> SITSSLDVRPEIKQAVTVRPGMCGPGSLFVGQLGDWTWETVSAQCDTDVFAARDASGNPTFLAFYYFRVRGGRELHPGSLTFGDRLTVTSGCYDQGTESVLTLHRIDRAGSDDAQRPLDLHEFYERPRDGSLYVENFNRWVTRSAPGSNEDLVKSSPPGFRNDGLPQLP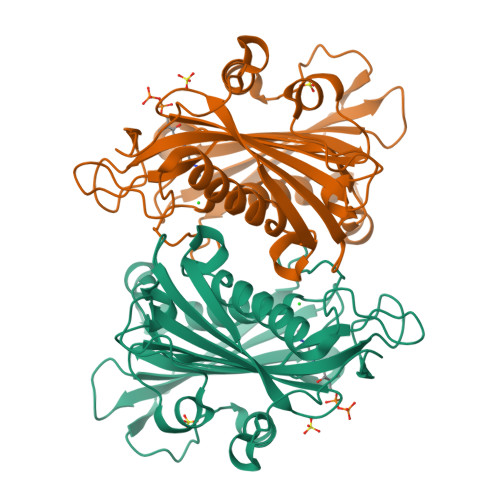AAYSPRAVYREARTAHTFRALDEPGFRLLPDTVEVEHPVDIVRDVNGVGLLYFASYFSMVDKAALALWRRLGRSDRAFLRRVVVDQQMCYLGNADLDSVLTLGARVRVSTETPGEELVDVVISDRDSGRVIAVSTLHTQHDAHDPKGEA> AMTRKQLINSMDMMRSACAPKFKVSTEMLDNLRGGIFAEDRELKCYTMCIAQMAGTMNKKGEINVQKTLAQMDAMLPPDMRDKAKEAIHSCRDVQGRYKDSCDKTFYSTKCLAEYDRDVF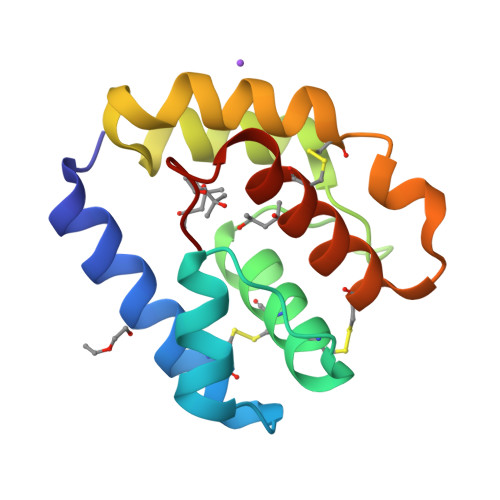LFP>[6x]GSHMASPNGQTKPLPALKLALEYIVPCMNKHGICVVDDFLGKETGQQIGDEVRALHDTGKFTDGQLVSQKSDSSKDIRGDKITWIEGKEPGCETIGLLMSSMDDLIRHCNGKLGSYKINGRTKAMVACYPGNGTGYVRHVDNPNGDGRCVTCIYYLNKDWDAKVSGGILRIFPEGKAQFADIEPKFDRLLF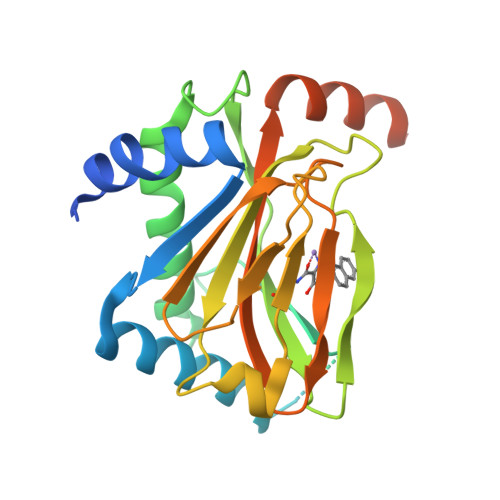FWSDRRNPHEVQPAYATRYAITVWYFDADERARAKVKYLTGEKGVRVELNKPSDSVGKDVF> XSLSAKDKANVKAIWGKILPKSDEIGEQALSRMLVVYPQTKAYFSHWASVAPGSAPVKKHGITIMNQIDDCVGHMDDLFGFLTKLSELHATKLRVDPTNFKILAHNLIVVIAAYFPAEFT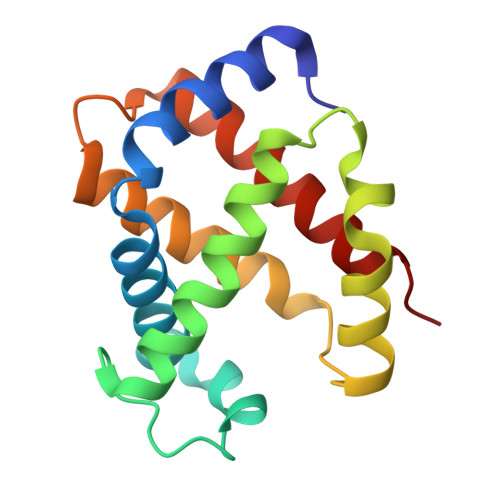PEIHLSVDKFLQQLALALAEKYR> MIPGANLLRMAFGVIGTQIVKYRKFEQRVKNDQAQYVSMFEEPFDLAASVQRVRRDQYVQFNLEFQRNYVMIF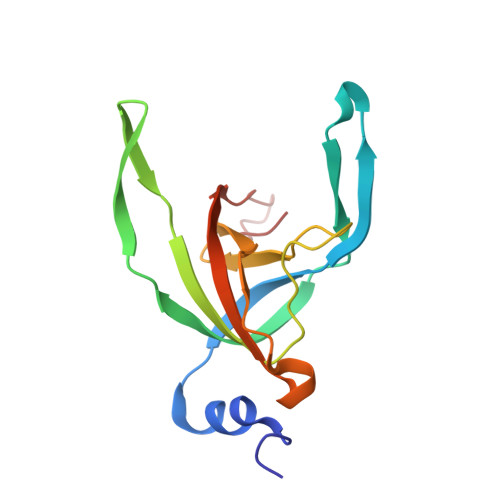ANFEMVDLDRDVAGDQFLWTGRVFQLESQGSWFYQDGWGVCLAVDIGAAKLTDDGKPTF> MAATTCFFFLFPFLLLLTLSRAATFEIVNRCSYTVWAAASKGDAALDAGGRQLNSGESWTINVEPGTKGGKIWARTDCYFDDSGSGICKTGDCGGLLRCKRFGRPPTTLAEFSLNQYGKDYIDISNIKGFNVPMDFSPTTRGCRGVRCAADIVGQCPAKLKAPGGGCNDACTVFQTSEYCCTTGKCGPTE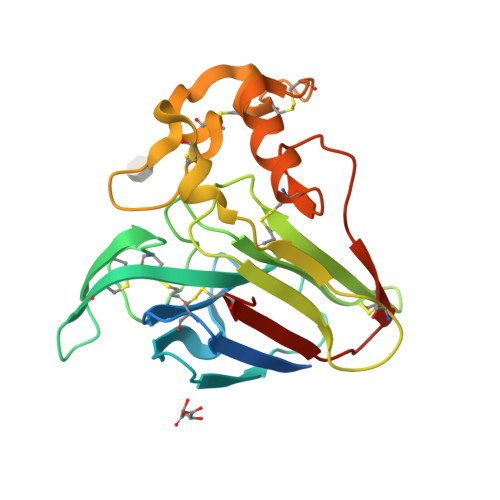YSRFFKRLCPDAFSYVLDKPTTVTCPGSSNYRVTFCPTALELEDE ethyl 4-[(2R)-2-(aminomethyl)morpholin-4-yl]-3-(3-cyanophenyl)-1H-pyrazolo[3,4-b]pyridine-5-carboxylate 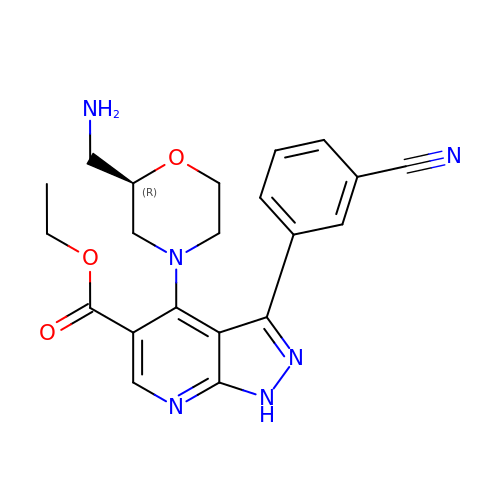| C21 H22 N6 O3 | XEAFNJRJCDEJPR-OAHLLOKOSA-N> HMKFRAKIVDGACLNHFTRISNMIAKLAKTCTLRISPDKLNFILCDKLANGGVSMWCELEQENFFNEFQMEGVSAENNEIYLELTSENLSRALKTAQNARALKIKLTNKHFPCLTVSVELLSMSSSSRIVTHDIPIKVIPRKLWKDLQEPVVPDPDVSIYLPVLKTMKSVVE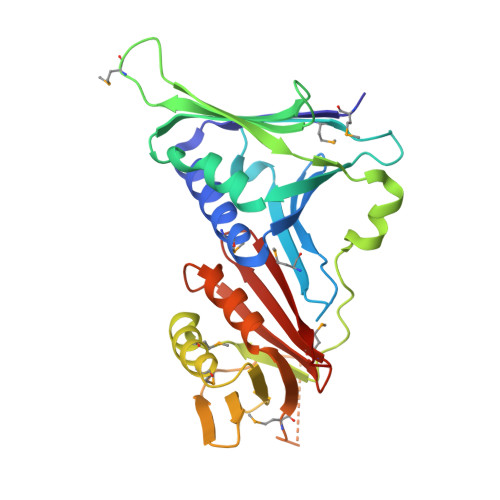KMKNISNHLVIEANLDGELNLKIETELVCVTTHFKDLGNPPLASESTHEDRNVEHMAEVHIDIRKLLQFLAGQQVNPTKALCNIVNNKMVHFDLLHEDVSLQYFIPALS> PNSLEAQIRQAMKTGSTLTIEFDQALNQKSPGTLNVFLHPANGGVRIDLDSGNQGEPAKILWLPWKQGELQTLQPGSISTVDMLFFTYYLSGSKVFAGDGGPVWHIDAPVEANQFWRRMSSDEWMEDWEVGTDRQVAYLHRAGQSDSLWNLSAYLEGA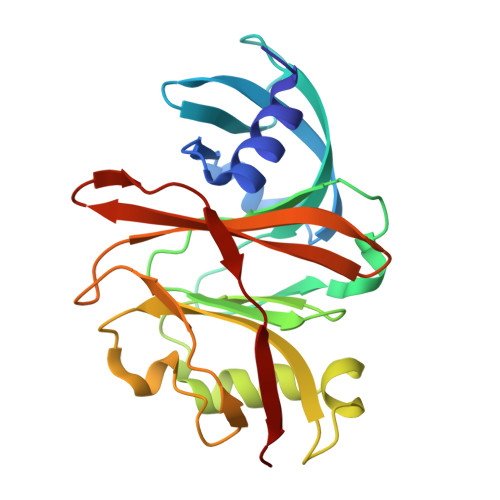APSTYGRDNLGQAVVGGIVTGRQQMSLYQYATTSSGSSAWSPLTYTLQQRKQ> FMVSLPRMVYPQPKVLTPCRKDVLVVTPWLAPIVWEGTFNIDILNEQFRLQNTTIGLTVFAIKKYVAFLKLFLETAEKHFMVGHRVHYYVFTDQPAAVPRVTLGTGRQLSVLEVRAYKRWQDVSMRRMEMISDFCERRFLSEVDYLVCVDVDMEFRDHVGVEILTPLFGTLHPGFYGSSREAFTYERRPQSQAYIPKDEGDFYYLGGFFGGSVQEVQRLTRACHQ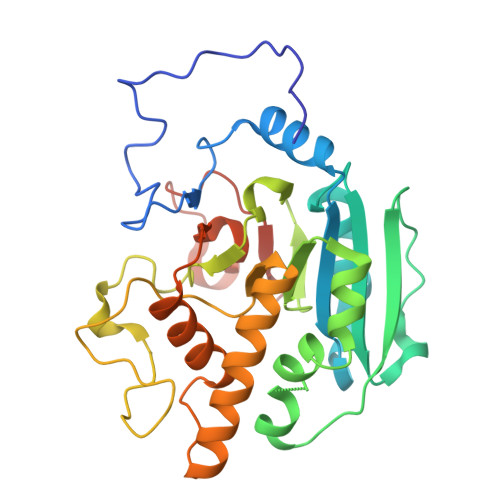AMMVDQANGIEAVWHDDSHLNKYLLRHKPTKVLSPEYLWDQQLLGWPAVLRKLRFTAVPKNHQAVRNPE> XTVFTSWEEYLDWV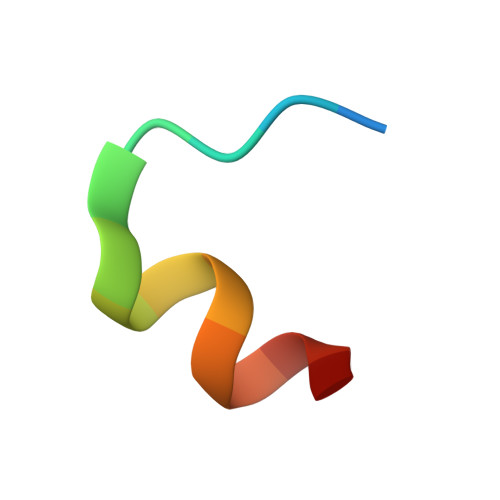X> AAQPAEALEDDGLCSADQKSCAQSEPDQINEDEFSFKIRRQIEKANADYKPCSSDPQDSDCSCHANVLKRDLAPYKSTGVTRQMIESSARYGTKYKIYGHRLYRDANCMFPARCEGIEHFLLPLVATLPDMDLIINTRDYPQLNAAWGNAAGGPVFSFSKTKEYRDIMYPAWTF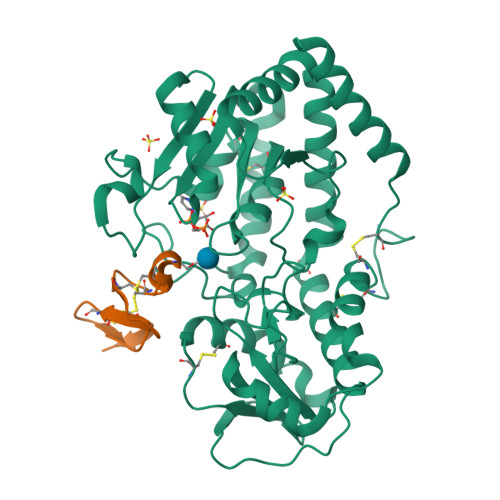WAGGPATKLHPRGIGRWDQMREKLEKRAAAIPWSQKRSLGFFRGSRTSDERDSLILLSRRNPELVEAQYTKNQGWKSPKDTLDAPAADEVSFEDHCKYKYLFNFRGVAASFRLKHLFLCKSLVFHVGDEWQEFFYDQLKPWVHYVPLKSYPSQQEYEHILSFFKKNDALAQEIAQRGYDFIWEHLRMKDIKCYWRKLLKRYVKLLQYEVKPEDQLIYIGPKARALVPR;> MDIVDGDQCESNPCLNGGSCKDDINSYECWCPFGFEGKNCELLEHHHHHH>GHHHHHHEFMHVFDNNGIELKAECSIGEEDGVYGLILESWGPGDRNKDYNIALDYIIERLVDSGVSQVVVYLASSSVRKHMHSLDERKIHPGEYFTLIGNSPRDIRLKMCGYQAYFSRTGRKEIPSGNRTKRI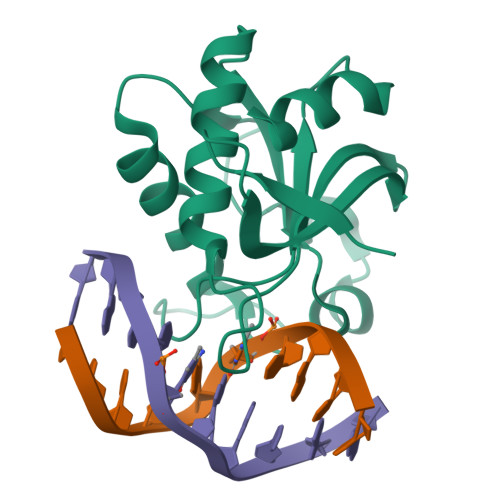LINVPGIYSDSFWASIIRG[2x]>GPHADGDQNLFDYQFTGTPEEPIKGYWTTTISYRDSKPKISLTIRQEFVEGGVESQAVLATVVGRPHLQDFLLLKRKHLEYSDYPESIDLIEFGDVKVIEKTV[2x]

The two genome segments code for four viral proteins, the nucleoprotein (NP), the glycoprotein-precursor, the small matrix protein Z and the large > 200 kDa L protein which harbors the viral RNA-dependent RNA polymerase. The L protein synthesizes two distinct RNA species: (i) the antigenomic and genomic RNA as products of genome replication and (ii) the shorter capped viral mRNAs during transcription. To initiate viral transcription, the L protein presumably uses a process called cap-snatching. It is assumed that the L protein cleaves host cell mRNAs downstream of the 5'-cap structure and uses this short capped RNA as a primer for viral mRNA synthesis. Here we present the crystal structures of the two terminal domains of the CASV L protein: the cap-snatching endonuclease in the N-terminus and the 326 C-terminal residues, which, by analogy to LASV, might play a role in transcription.

To further substantiate that L-Cterm domain 1 has no influence on the conformation of L-Cterm domain 2, we crystallized and solved the structure of the isolated domain 2. This structure was refined to a resolution of 1.8 Å. CASV L-Cterm domain 2 also crystallized as a dimer but—due to absence of domain 1—with a completely different and much smaller interface compared to CASV L-Cterm. The protein also appeared as a dimer in solution as shown by SAXS. Superimposition of the isolated Cterm domain 2 with its counterpart in the full CASV L-Cterm structure shows only small differences in the loop upstream of W1818 and no major rearrangement of potential cap-binding side chains, even though B-factors are relatively high around the putative cap-binding site. Co-crystallization of the domain with m7GpppG, m7GTP, GTP or ATP did not result in additional electron density. Again, we did not detect binding to m7GTP-agarose of the isolated CASV L-Cterm domain 2 nor a thermal stabilization of the protein by m7GTP. We detected a shift of the RNA with PB2, but not with L-Cterm domain 2. As neither a monomeric form of CASV L-Cterm (deltaC) nor a dimeric form with a different dimer interface (domain 2) binds m7GTP, we conclude that the dimerization of the protein and the presence of domain 1 are not responsible for the lack of cap-binding activity.> GSEFQNKNFRAPQSEAIGILYKLIETGSKHKNMYDHTEITTDSLLALLGSEKVKIIDVRSADAYNGWRMRGEVRGGHIKGAKSLPAKWLTDPEWLNIVRFKQIRPEDAIVLYGYTPEECEQTATRFKENGYNNVSVFHRFHPDWTGNDAFPMDRLEQYNRLVPAEWVNGLISGEEIPEYDNDTFIVCHAHYRNRDAYLSGHIPGATDMDTLALESPETWNRRTPEELKKALEEHGITASTTVVLYGKFMHPDNADEFPGSA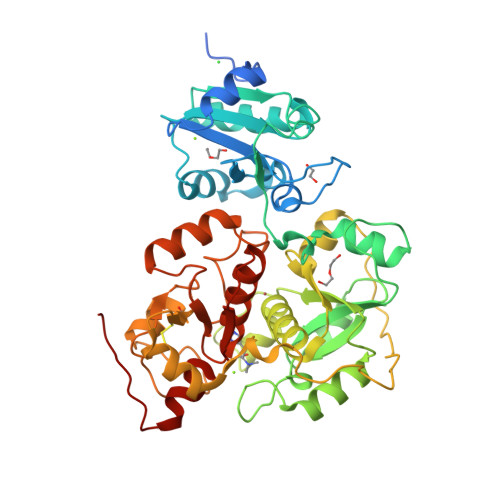AGHIGAIRLAFIMMYAGVEDVRVLNGGYQSWTDAGFAISKDDVPKTTVPEFGAPIPSRPEFAVDIDEAKEMLQSEDSDLVCVRSYPEYIGEVSGYNYIKKKGRIPGAIFAECGSDAYHMENYRNHDHTTREYHEIEDIWAKSGIIPKKHLAFYSGTGWRGSEAWFNALLMGWPRVSVYDGGWFEWSNDPENPYETGVPK> MKHHHHHHGKA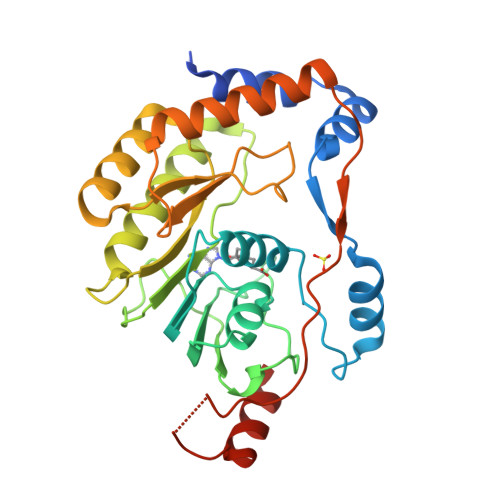AGVTLGEVWKRQLNMLGKQEFERYKVSDITEVDRTAARRYLKEGRTDVGISVSRGAAKIRWLHERGYLRITGRVLDLGCGRGGWSYYAAAQKEVMSVKGYTLGIEGHEKPIHMQTLGWNIVKFKDKSNVFTMPTEPSDTLLCDIGESSSNPLVERDRTMKVLENFERWKHVNTENFCVKVLAPYHPDVIEKLERLQLRFGGGIVRVPFSRNSTHEMYYISGARNNITHMVNTTSRSLLRRMTRPSGKAIIEGDVFLPTGTRSVASEAGTIDHEALKLRVDQIKAEYSKT>SLINTKIKPFKNQAFKNGEFIEVTEKDTEGRWSVFFFYPADFTFVCPTELGDVADHYEELQKLGVDVYSVSTDTHFDHKAWHSSSETIAKIKYAMIGDPTGALTRNFDNMREDEGLADRATFVVDPQGIIQAIEVTAEGI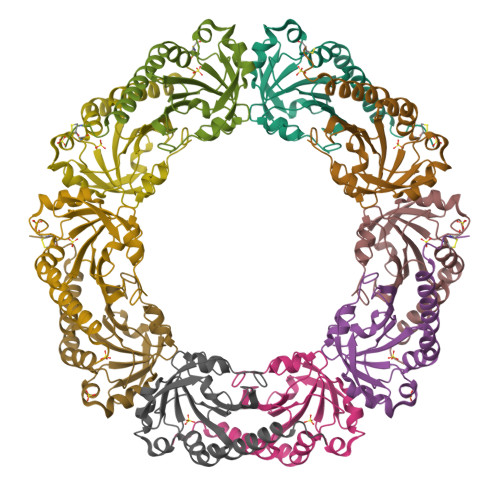GRDASDLLRKIKAAQYVAAHPGEVCPAKWKEGEATLAPSLDLVGKI[5x]>[2x]GSHMEKLAKNKVISIDAGRKYFTLNQLKRIVDKASELGYSDVHLLLGNDGLRFLLDDMTITANGKTYASDDVKKAIIE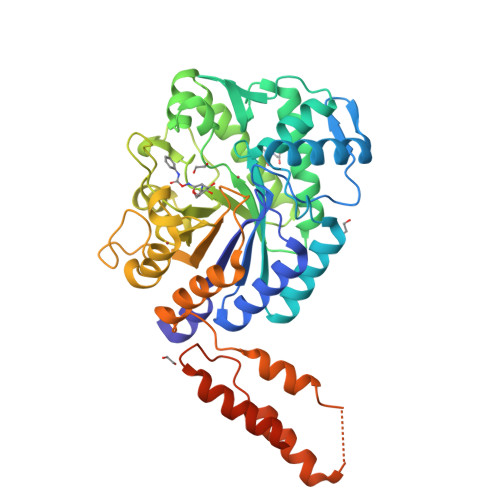GTKAYYDDPNGTALTQAEVTELIEYAKSKDIGLIPAINSPGHMDAMLVAMEKLGIKNPQAHFDKVSKTTMDLKNEEAMNFVKALIGKYMDFFAGKTKIFNFGTDEYANDATSAQGWYYLKWYQLYGKFAEYANTLAAMAKERGLQPMAFNDGFYYEDKDDVQFDKDVLISYWSKGWWGYNLASPQYLASKGYKFLNTNGDWYYILGQKPEDGWYFLKKAIENTGKTPFNQLASTKYPEVDLPTVGSMLSIWADRPSAEYKEEEIFELMTAFADHNKDYFRANYNALREELAKIPTNLEGYSKESLEALDAAKTALNYNLNRNKQAELDTLVANLKAALQGLKPAVTHSGSLDENEVAANVETRP>MEIKLQGKVSLVTGSTRGIGRAIAEKLASAGSTVIITGTSGERAKAVAEEIANKYGVKAHGVEMNLLSEESINKAFEEIYNLVDGIDILVNNAGITRDKLFLRMSLLDWEEVLKVNLTGTFLVTQNSLRKMIKQRWGRIVNISSVVGFTGNVGQVNYSTTKAGLIGFTKSLAKELAPRNVLVNAVAP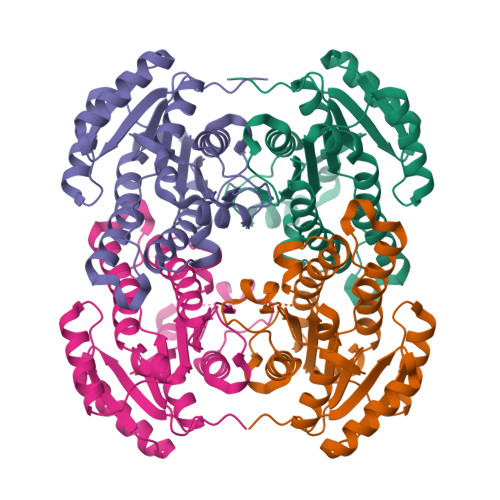GFIETDMTAVLSEEIKQKYKEQIPLGRFGSPEEVANVVLFLCSELASYITGEVIHVNGGMF[2x]>[2x]SPSINVALKAAFPSPPYLVELLETAASDNTTIYYSLLDRIAKGHFAEATTDKALYEKFLEVLRDDGHMDPEALSAFKLALSLRTATPRVEAHYQYYTATVEPSLSGTQEGCDQWFLIDGEQYCSPTLDTSHGKVKGEDQLRTLPFDRKFCVGSRDVILYADITSKSFAPFHEVAMDLAKKGKASYRVRYRRSPSHSRESLSVNGYGVELVLKRTDYIVIDDRDTGAAAKPAEENDQKPLVGHETVLDDGEEIADIKPLEKSELAALGMKAASFVMQSEKPFEALLKLTQDFPKYSNSLGSQNVSAEFEAEHRGNREVFLPEGSNVLWLNGLHLIDRQIQPFGLVDLLTRERKLIKSVLDLGLTGQQAVDLLGHAEVAHAKSGDDEPRRFDWRDDIEEGQVIIWLNNLEKDKRYKSFSPSIWVLIHHFGHGLPQIRRDVFNLVVPVDLTKADDVKIVVEGLLSFVKRLIPVRFGFVPLTPTGQAIDQAKVVYYLLENYGLAAATAYLEKSYEEQSTGQPNERIFNEVIKDKSLRPDGVELSFKDIFISEKHEKQIHLSKHWVERLRAGGDVPTVFFDGFPIPREDNWLRVMNHRLMQDLQALQQAGYFGMLNESMWLPGFFLEKALSRRNTLIFPEDKNELTVLNVNKIYIENHDLMSKVPVIEASKESTRDDWAALTVVADLDDIEGQELVYYALRFRKSNDGVRLDIVHNPKDTSRSPSVLAQRLKSREDKLLDFTRFLDLETALETGEFEPDVAYDCSLANFLASSNMKAGDNFVILNGRVLGPITSADDFKKEDFEVFLQAERRTRILPVYKALEDLGLDDKVSGPLSAAKLTSVTALSTISDLPQGIFDNAPTVRTTLFKQWNSTYTSFEVGDASTATIFFVAVINPASEIGQRWVAVLKVLSELEGVHLRVFLNPTVMIEELPVKRFYRYVLSSSPSFDESGKVKALSARFTGVPRETLLVVGMDVPPAWLVTSKVAVDDLDNLRIKDIKAKRGTEHVEAIYELEHILIEGHSREIPGAHAPRGVQLVLETENNPHFADTIIMANLGYFQFKANPGVYNIRLKEGRSSEIFTLESVGAKGWGPIPGDDNTEVVLMDFQGTTLYPRLRRKPGMEEEDVLEPSTKSGEESGSGARNLVSRGIKFAEGLLGRGNKAAEATKSVSKTEHAEINIFSVASGHLYERMLNIMMASVMHHTNHTVKFWFIEQFLSPSFKDFIPHMAAEYGFKYEMVTYKWPHWLRQQKEKQREIWGYKILFLDVLFPLSLDKVIFVDADQIVRTDMYDLVEHPLDGAPYGFAPMCDSRVEMEGYRFWKTGYWANYLKGKPYHISALYVVDLQRFRELAAGDRLRQQYHALSADPNSLANLDQDLPNHMQFTIPI

Central to ERQC is the ER-resident 170-kDa enzyme UDP-glucose:glycoprotein glucosyltransferase (UGGT). The enzyme selectively reglucosylates a misfolded glycoprotein on one of its N-glycans and promotes its association with the ER lectins calnexin and calreticulin, thus mediating its ER retention. The full-length Chaetomium thermophilum UGGT (CtUGGT) crystal structures revealed four DsbA-like domains (TRXL1–4) arranged in a long arc, terminating in two β sandwiches (βS1 and βS2) tightly clasping the glucosyltransferase family 24 (GT24) domain (Roversi et al., 2017). Overall, UGGT's motions can be described in simple terms as two rigid groups of domains moving with respect to one another.

To probe the functional role of the “clamping” motion uncovered in the present analysis, we engineered four double-cysteine CtUGGT mutants, CtUGGTG178C/A786C, CtUGGTG177C/A786C, CtUGGTG179C/T742C, and CtUGGTS180C/T742C, all designed to form disulfide bridges across the TRXL1 and TRXL3 domains, clamping shut the cleft between them. The presence of the engineered disulfide bridges in the remaining three mutants was confirmed by mass spectrometry. The crystal structures of CtUGGTG177C/A786C and CtUGGTS180C/T742C were determined to about 4.6-Å resolution. Both crystal structures show the TRXL3 domain tethered to the TRXL1 domain by the extra disulfide bridge. We tested the in vitro activity of the three “clamped-shut” double Cys mutants (in addition to the activity of the wild type and the already published CtUGGTD611C/G1050C) on urea-misfolded bovine thyroglobulin. As to the UGGT clamping motion, we tested two a priori rather similar double-cysteine mutants, CtUGGTS180C/T742C and CtUGGTG177C/A786C, both designed to clamp the TRXL1-TRXL3 domains shut. Surprisingly, the two mutants differ in their ability to reglucosylate urea-misfolded bovine thyroglobulin, with the former mutant more active than (and the latter mutant having similar activity to) wild-type CtUGGT. These observations point to the possibility that each misfolded glycoprotein substrate may depend to a different degree on a different subset of UGGT inter-domain conformational degrees of freedom. The three motions are to some extent independent of each other. These observations open the way to the cloning, expression, and purification of Cys quadruple mutants such as CtUGGTG177C/A786C, D611C/G1050C: these mutants would block the molecule in a clamped and bent closed conformation across the cleft and the central saddle, respectively.>[2x]MADDQGCIEEQGVEDSANEDSVDAKPDRSSFVPSLFSKKKKNVTMRSIKT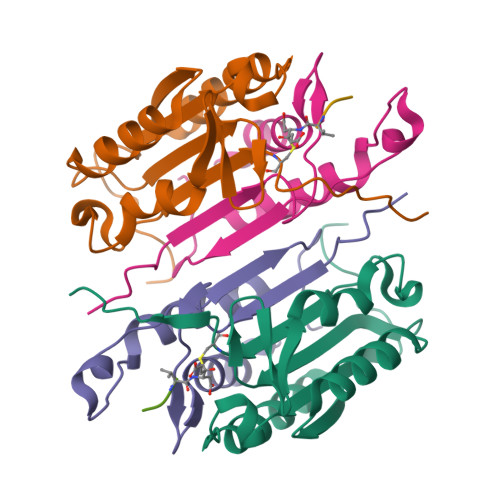TRDRVPTYQYNMNFEKLGKCIIINNKNFDKVTGMGVRNGTDKDAEALFKCFRSLGFDVIVYNDCSCAKMQDLLKKASEEDHTNAACFACILLSHGEENVIYGKDGVTPIKDLTAHFRGDRCKTLLEKPKLFFIQACRGTELDDGIQAD;>SGPINDTDANPRYKIPVEADFLFAYSTVPGYYSWRSPGRGSWFVQALCSILEEHGKDLEIMQILTRVNDRVARHFESQSDDPHFHEKKQIPCVVSMLTKELYFSQLEHHHHHH[2x]> MNDIAHNLAQVRDKISAAATRCGRSPEEITLLAVSKTKPASAIAEAIDAGQRQFGENYVQEGVDKIRHFQELGVTGLEWHFIGPLQSNKSRLVAEHFDWCHTIDRLRIATRLNDQRPAELPPLNVLIQINISDENSA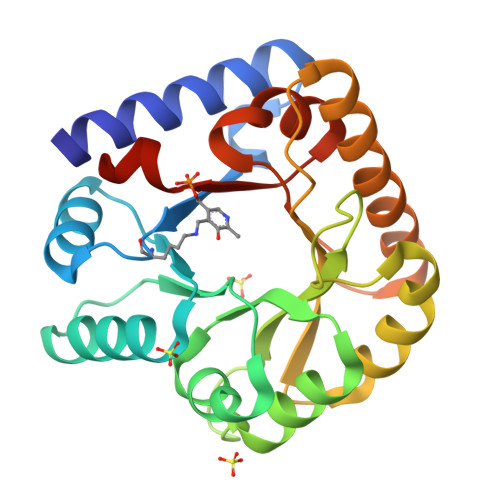SGIQLAELDELAAAVAELPRLRLRGLMAIPAPESEYVRQFEVARQMAVAFAGLKTRYPHIDTLSLGMSDDMEAAIAAGSTMVRIGTAIFGARDYSKK> MAAACRSVKGLVAVITGGASGLGLATAERLVGQGASAVLLDLPNSGGEAQAKKLGNNCVFAPADVTSEKDVQTALALAKGKF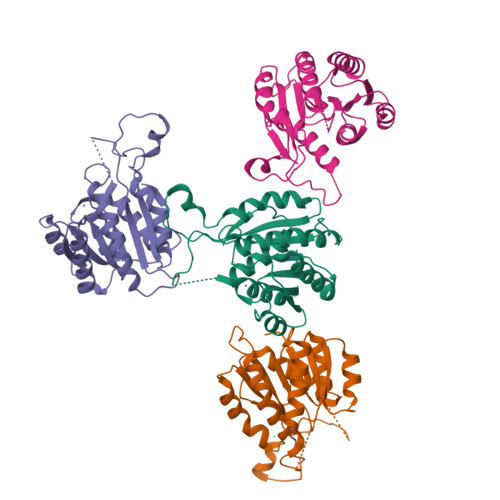GRVDVAVNCAGIAVASKTYNLKKGQTHTLEDFQRVLDVNLMGTFNVIRLVAGEMGQNEPDQGGQRGVIINTASVAAFEGQVGQAAYSASKGGIVGMTLPIARDLAPIGIRVMTIAPGLFGTPLLTSLPEKVCNFLASQVPFPSRLGDPAEYAHLVQAIIENPFLNGEVIRLDGAIRMQP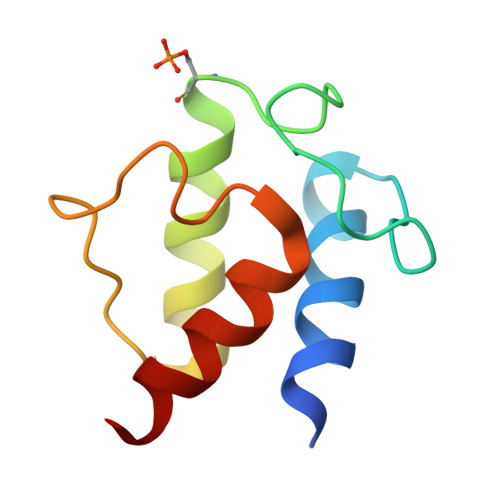> GSHMDVKAEVIEIIDELFMEDVSDMMDEDLFDAGVLDSMGTVELIVELESRFDIRVPVSEFGRDDWNTANKIVEGVTELRNA> EDLLKNLLTMGVDIDMARKRQPGVFHRMITNEQDLKMFLLSKGASKEVIASIISRYPRAITRTPENLSKRWDLWRKIVTSDLEIVNILERSPESFFRSNNNLNLENNIKFLYSVGLTRKCLCRLLTNAPRTFSNSLDLNKQMVEFLQAAGLSLGHNDPADFVRKIIFKNPFILIQSTKRVKANIEFLRSTFNLNSEELLVLICGPGAEILDLSNDAARRSYANIKEKLFSLGCTEEEVQKFVLSYPDVIFLAEKKFNDKIDCLMEENISISQIIENPRVLDSSISTLKSRIKELVN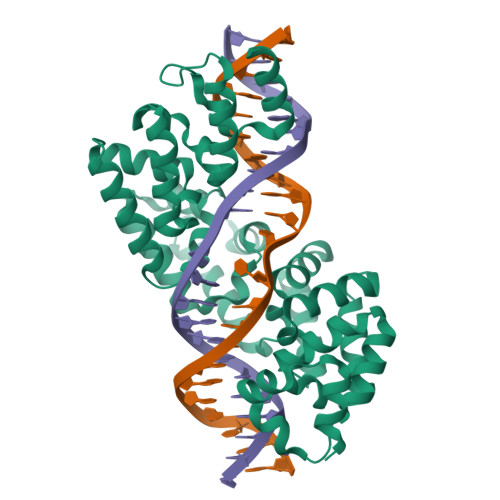AGCNLSTLNITLLSWSKKRYEAKLKKLS>[2x]MLGQMMTQPLLISSLIDHAARYHGQTEIVSVETDGTVTRTNWGEIAANARRMGSALTKLGLQPQDRIGTLAWNNRRHLEIYYAASGAGFVCHTINPRLFPEQLVYIINHAQDRVLFFDATFLPLVAAIRDQLTEVKHFVLMGPRNEDALQQ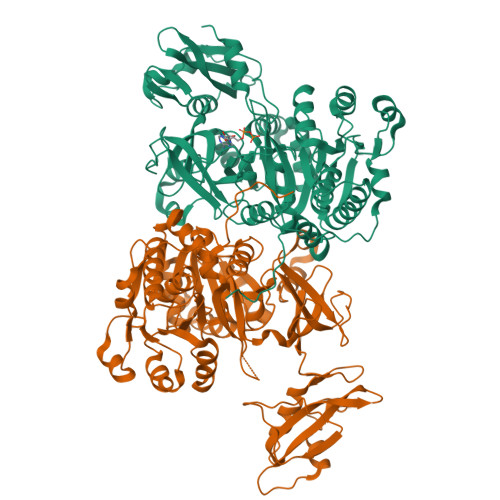IPGLEFYDELIETGDTDFEWPVFDENTASSLCYTSGTTGHPKGVLYSHRSTVLHSFASNTRDVIGYSAMDVVMPVVPMFHVNAWGSPYGCAMSGAQMVLPGPDLHGEALVNLIDTYGVTLAMGVPTIWQGLLAHAAKCGTKLESLERTVIGGAACPPSMIATFREKYGVDTVHAWGMSEMSPLGTANIPLAKHRKLPIEEQHKLRENQGRPPFGVELKIVDDDGNDLPHDGVTQGDLMVRGHWVLDSYFQLKDQELLQDGWFATGDVATLDPDGYMTIRDRSKDIIKSGGEWISSVELENIAVAHPKLATAAVIGVPHPKWDERPLLVAVKAEGEDPSEAELLEFFDGKIAKWQVPDKVVFVDALPLNATGKVLKRKLRDEFKDALTG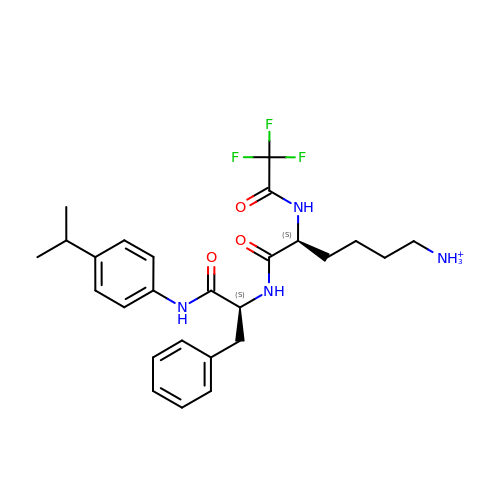6-ammonio-N-(trifluoroacetyl)-L-norleucyl-N-[4-(1-methylethyl)phenyl]-L-phenylalaninamide | C26 H34 F3 N4 O3 | SKWCLCMPIGFAOR-VXKWHMMOSA-O> MPFVNKQFNYKDPVNGVDIAYIKIPNAGQMQPVKAFKIHNKIWVIPERDTFTNPEEGDLNPPPEAKQVPVSYYDSTYLSTDNEKDNYLKGVTKLFERIYSTDLGRMLLTSIVRGIPFWGGSTIDTELKVIDTNCINVIQPDGSYRSEELNLVIIGPSADIIQFECKSFGHEVLNLTRNGYGSTQYIRFSPDFTFGFEESLEVDTNPLLGAGKFATDPAVTLAHQLIHAGHRLYGIAINPNRVFKVNTNAYYEMSGLEVSFEELRTFGGHDAKFIDSLQENEFRLYYYNKFKDIASTLNKAKSIVGTTASLQYMKNVFKEKYLLSEDTSGKFSVDKLKFDKLYKMLTEIYTEDNFVKFFKVLNAKTFLNFDKAVFKINIVPKVNYTIYDGFNLRNTNLAANFNGQNTEINNMNFTKLKNFTGLFEFYKLLCVRGIITSKTKSLDKGYNKALNDLCIKVNNWDLFFSPSEDNFTNDLNKGEEITSDTNIEAAEENISLDLIQQYYLTFNFDNEPENISIENLSSDIIGQLELMPNIERFPNGKKYELDKYTMFHYLRAQEFEHGKSRIALTNSVNEALLNPSRVYTFFSSDYVKKVNKATEAAMFLGWVEQLVYDFTDETSEVSTTDKIADITIIIPYIGPALNIGNMLYKDDFVGALIFSGAVILLEFIPEIAIPVLGTFALVSYIANKVLTVQTIDNALSKRNEKWDEVYK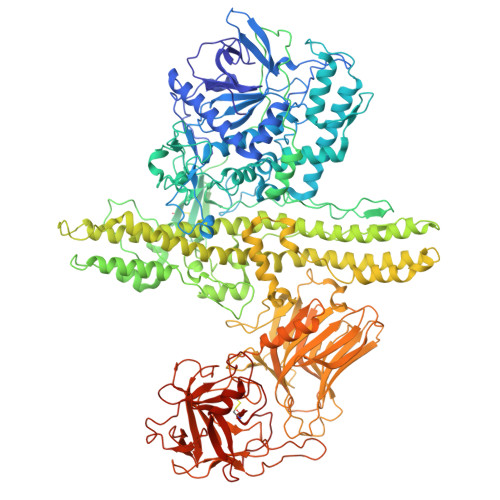YIVTNWLAKVNTQIDLIRKKMKEALENQAEATKAIINYQYNQYTEEEKNNINFNIDDLSSKLNESINKAMININKFLNQCSVSYLMNSMIPYGVKRLEDFDASLKDALLKYIYDNRGTLIGQVDRLKDKVNNTLSTDIPFQLSKYVDNQRLLSTFTEYIKNIINTSILNLRYESNHLIDLSRYASKINIGSKVNFDPIDKNQIQLFNLESSKIEVILKNAIVYNSMYENFSTSFWIRIPKYFNSISLNNEYTIINCMENNSGWKVSLNYGEIIWTLQDTQEIKQRVVFKYSQMINISDYINRWIFVTITNNRLNNSKIYINGRLIDQKPISNLGNIHASNNIMFKLDGCRDTHRYIWIKYFNLFDKELNEKEIKDLYDNQSNSGILKDFWGDYLQYDKPYYMLNLYDPNKYVDVNNVGIRGYMYLKGPRGSVMTTNIYLNSSLYRGAKFIIKKYASGNKDNIVRNNDRVYINVVVKNKEYRLATNASQAGVEKILSALEIPDVGNLSQVVVMKSKNDQGITNKCKMNLQDNNGNDIGFIGFHQFNNIAKLVASNWYNRQIERSSRTLGCSWEFIPVDDGWGERPLVPPTPGSAWSHPQFEK> MHFEAYPPEVNSANIYAGPGPDSMLAAARAWRSLDVEMTAVQRSFNRTLLSLMDAWAGPVVMQLMEAAKPFVRWLTDLCVQLSEVERQIHEIVRAYEWAHHDMVPLAQIYNNRAERQILIDNNALGQFTAQIADLDQEYDDFWDEDGEVMRDYRLRVSDALSKLTP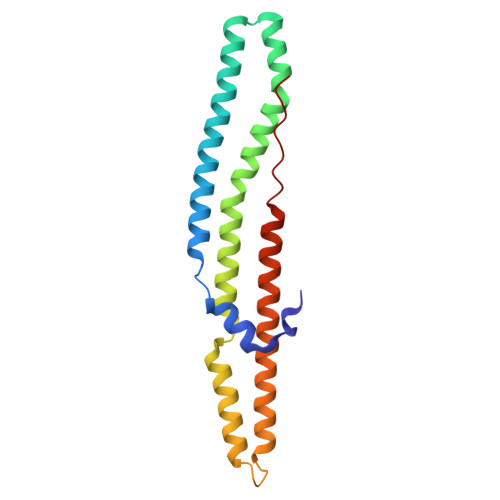WKAPPPIA>[4x]HHHHHHSSGLVPR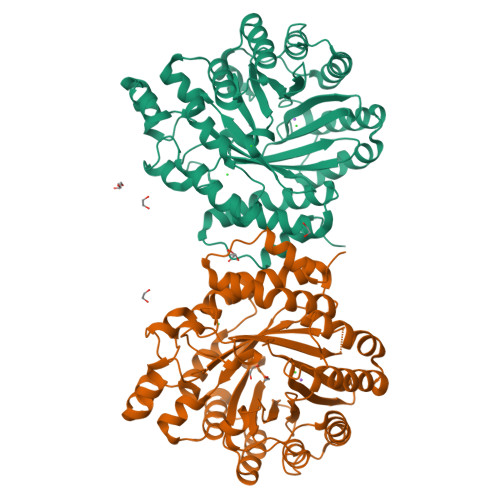GSHQSQAPIPKDIAYHTLTKALLFPDIDQYQHWHHVAPMLAKMLVDGKYSIHQQYEYLCLFAQLVAPVLGPYPSPGRDVYRCTLGGNMTVELSQNFQRSGSTTRIAFEPVRYQASVGHDRFNRTSVNAFFSQLQLLVKSVNIELHHLLSEHLTLTAKDERNLNEEQLTKYLTNFQVKTQYVVALDLRKTGIVAKEYFFPGIKCAATGQTGSNACFGAIRAVDKDGHLDSLCQLIEAHFQQSKIDDAFLCCDLVDPAHTRFKVYIADPLVTLARAEEHWTLGGRLTDEDAAVGLEIIRGLWSELGIIQGPLEPSAMMEKGLLPIMLNYEMKAGQRLPKPKLYMPLTGIPETKIARIMTAFFQRHDMPEQAEVFMENLQAYYEGKNLEEATRYQAWLSFAYTKEKGPYLSIYYFWPE The simplest TCSs comprise a sensory histidine kinase (HK) and a response regulator (RR) component. To address this question we have used the TCS DesK-DesR from B. subtilis as a model. We had previously shown that the HK DesK, a member of the HisKA_3 family, undergoes important conformational changes to switch between phosphatase- and phosphotransfer-competent states. We now report the crystal structures of the DesKC:DesR complex, trapped in the phosphatase and the phosphotransferase functional states.

One using the phosphatase-constitutive mutant DesKCSTAB, and the other with DesKCH188E carrying a phosphomimetic substitution, both in complex with the REC domain of DesR. (D) Cartoon representation of the DesKCH188E:DesR-REC (phosphotransferase) complex, along two orthogonal views (left and right subpanels). Note best fitting with a one dimer DesKCH188E (chains AB) to one monomer DesR-REC (chain C) model. The structures show the RR REC domain adopting identical conformations in both phosphatase and phosphotransferase complexes, presenting active- and inactive–like features in different regions of the protein, arranging the RR’s active site for phosphoryl group migration. Except for the phosphate lid, the REC domain bound to the HK largely resembles the RR’s active form, shifting the position of the β1α1 loop and helix α1, now able to recruit the Mg2+ cation essential for phosphoryl-transfer catalysis. The β4α4 loop in DesR plays a key role in these controls, remodeling its configuration in concert with DesK-association. This loop, acting as a phosphate lid, is open in the phosphotransferase complex, enabling the transfer reaction. Taking into account that phosphotransfer is a nucleophilic substitution at phosphorus, the reaction coordinate distance (i.e. between phosphorus and the entering atom, before the transfer reaction has begun) strongly suggests that P~DesK→DesR phosphotransfer occurs through a largely dissociative, or ‘loose’ mechanism: a reaction coordinate distance of ≥4.9 Å provides room for a fully dissociated metaphosphate intermediate. Our model predicts an important role of the highly conserved Thr80(RR) in stabilizing an intermediary metaphosphate group, ideally positioned to accompany the migrating phosphoryl moiety. Yet, the phosphate lid is expected to close in, following the phosphoryl migration during transfer, due to the strong phosphoryl-Thr80(RR) interaction. Phosphotransfer thus results in a fully activated RR configuration, with a closed phosphate lid that ensures the release of a stable P~DesR species, as observed in active free RR structures.

>[4x]GRKERERLEEKLEDANERIAELVKLEERQRIARDLEDTLGQKLSLIGLKSDLARKLIYKDPEQAARELKSVQQTARTSLNEVRKIVSSMKGIRLKDELINIKQILEAADIMFIYEEEKWPENISLLNENILSMCLKEAVTNVVKHSQAKTCRVDIQQLWKEVVITVSDDGTFKGEENSFSKGHGLLGMRERLEFANGSLHIDTENGTKLTMAIPNNSK;>GSGSMISIFIAEDQQMLLGALGSLLNLEDDMEVVGKGTTGQDAVDFVKKRQPDVCIMDIEMPGKTGLEAAEELKDTGCKIIILTTFARPGYFQRAIKAGVKGYLLKDSPSEELANAIRSVMNGKRIYAPELMEDLYSEA[2x]>MSSRVSTRSSLAEDLRAIGLADGDAVLVHAALRKVGKIVGGPDDILDAMRDVIGPAGTVLGYADW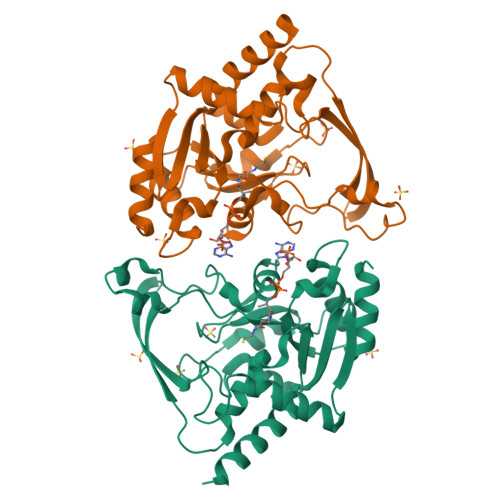QLEDEIRDDPAMREHIPAFDPLRSRSIRDNGFWPELIRTTPGALRSASPGASMAAIGGEAEWFTADHALDYGYGPRSPLGKLVEAKGKVLMLGAPLDTMTLLHHAEHLADFPNKRILRYEAPILVDGEKVWRWFEEFDTSDPPDGLADDYFAGIVEEFLATGRGKRGKIGEASSVLVPADEIVAFAVDWLERWGRTAR[6x]> SPSGSTIEAGIAYPISTGFDPLTSSGASSMAANLHIFEGLVDLHPVTRQPYLALAAKEPEQKDDLTYYISLREGAMFHDGSPVTTEDVVYSFERVLDPAKASLFAQFIPFIASVTALDDNVVEFKLKYPFALFKERLTIIKIVPKHIVEAGQSAFDAKPIGSGPYKFVSATKDDRIVFEANTVYNGHYPAKVEKMTWFLLSDDAARVTAQESGRVQAIESVPYLDAERLKRKNNVESVQSFGLLFLMFNCEKAPFDNPKVRQALHYALDKQKLIDIVFLGNAKAATSYLQDTHPDYVKASSQYDYDKAKAEKLLAEAGITNLTFQLLATDHAWVKECAPLILESWNALSVVKVTLQHLQSGALYSAHVDKGAYEVVIAPGDPSVFGNDLDL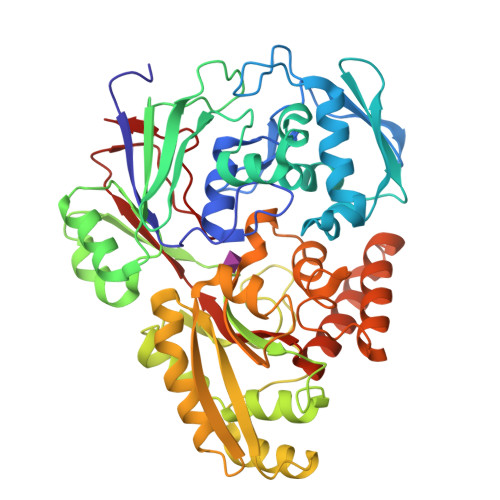LLSWWYRGDVWPKRRFRWANTAEYHEVQKLLDEAIKNPAGSKVAWQKAINIIAEQVPLYPIIHRKLPTAWNTKKLTDFQPLPTTGLSFLGVGRT> QFLFSMSTGPFICTVKDNQVFVANLPWTMLEGDDIQVGKEFAARVEDCTNVKHDMAPTCTKPPPFCGPQDMKMFNFVGCSVLGNKLFIDQKYVRDLTAKDHAEVQTFREKIAAFEEQQENQPPSSGMPHGAVPAGGLSP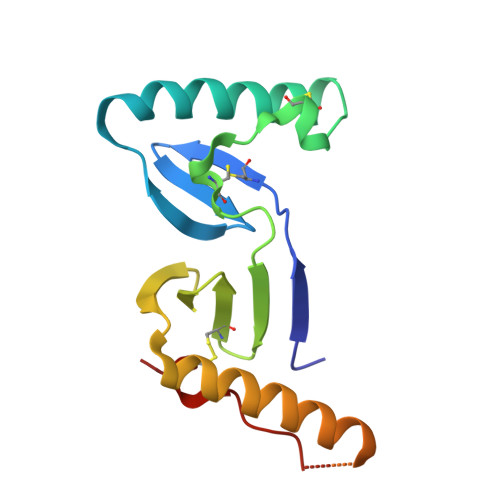PPPPSFCTVQ>MAEQVALSRTQVCGILREELFQGDAFHQSDTHIFIIMGASGDLAKKKIYPTIWWLFRDGLLPENTFIVGYARSRLTVADIRKQSEPFFKATPEEKLKLEDFFARNSYVAGQYDDAASYQRLNSHMNALHLGSQANRLFYLALPPTVYEAVTKNIHESCMSQIGWNRIIVEKPFGRDLQSSDRLSNHISSLFREDQIYRIDHYLGKEMVQNLMVLRFANRIFGPIWNRDNIACVILTFKEPFGTEGRGGYFDEFGIIRDVMQNHLLQMLCLVAMEKPASTNSDDVRDEKVKVLKCISEVQANNVVLGQYVGNPDGEGEATKGYLDDPTVPRGSTTATFAAVVLYVENERWDGVPFILRCGKALNERKAEVRLQFHDVAGDIFHQQCKRNELVIRVQPNEAVYTKMMTKKPGMFFNPEESELDLTYGNRYKNVKLPDAYERLILDVFCGSQMHFVRSDELLEAWRIFTPLLHQIELEKPKPIPYIYGSRGPTEADELMKRVGFQYEGTYKWVNPHKL[8x]

Reduced glutathione (GSH) provides the cellular first line of defense against oxidative stress-induced injury, which can be maintained by NADPH generated mainly via the pentose phosphate pathway and its rate-limiting enzyme, glucose-6-phosphate dehydrogenase (G6PD). Accordingly, missense DNA mutations that impair G6PD activity or stability result in increased oxidative stress and a spectrum of disease phenotypes featuring, most commonly, hemolytic anemia, and collectively called G6PD deficiency. Each monomer has a catalytic nicotinamide adenine dinucleotide phosphate (NADP+)-binding domain and β+α domain, containing an additional binding site for NADP+ that structurally stabilizes the enzyme. The glucose 6-phosphate (G6P)-binding site is located between these two domains.

We first began our efforts focusing on the Canton variant, with the mutation R459L, located in the β+α domain. Canton G6PD is prevalent in China and Southeast Asia (50–60% of the variants), causing severe deficiency (class II). Recombinant Canton G6PD enzyme showed only 18% of normal G6PD activity with lower KM for both NADP+ and G6P, which is consistent with the biochemical characteristics analyzed using blood samples derived from subjects carrying the Canton variant. Furthermore, the Canton variant was less thermostable; its T1/2, the temperature at which the enzyme retains half of its catalytic activity, was 42.6 °C, which is 4.6 °C lower than T1/2 of WT enzyme. To elucidate the molecular basis of the reduced stability and activity of Canton G6PD, we examined the crystal structures of WT and Canton G6PD at 1.9 Å and 2.6 Å resolution, respectively. Although no NADP+ was added to protein solution prior to the crystallization, both crystal structures contained NADP+ at the second NADP+-binding site (structural NADP+-binding site) in the β+α domain. However, we noticed a loose helical interaction between the helix (αn), containing the Canton variant-R459L, and an adjacent helix (αe), which was not described in previously reported structures. In WT G6PD, R459 forms electrostatic and hydrogen bond interactions with D181 and N185 on the adjacent helix (αe), whereas Canton mutation does not, resulting in loosened inter-helical interactions and displacements of the helix (αe) and a proceeding loop consisting of K171, P172, F173, G174, and R175, several amino acids away from R459-interacting residues on the helix (αe). Thus, the loose inter-helical interaction in the Canton variant is likely to be a major driving force for positioning the loop and thus changing the orientations of these residues. Canton G6PD was more susceptible to degradation by chymotrypsin relative to the WT enzyme, which corresponded with a significantly decreased enzymatic activity. This suggests that Canton G6PD may undergo higher conformational fluctuation, leading to a greater accessibility to proteases and its reduced thermostability.>[2x]GSWFHEGLSRHQAENLLMGKEVGFFIIRASQSSPGDFSISVRHEDDVQHFKVMR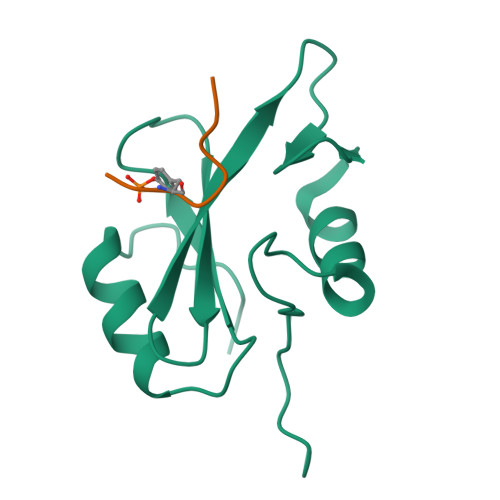DNKGNYFLWTEKFPSLNKLVDYYRTNSISRQKQIFLRDRTREDQGH;>[2x]SDYMNMTP First structural insight into lipid scrambling was provided from the X-ray structure of the fungal protein from Nectria haematococca, termed nhTMEM16. This protein is part of the TMEM16 family, which encompasses calcium-activated ion channels and lipid scramblases with a conserved molecular architecture. As common for the family, nhTMEM16 is a homodimer with subunits containing a cytoplasmic domain and a transmembrane unit composed of 10 membrane-spanning segments. The lipid permeation path is defined by a structural entity termed the ‘subunit cavity’, which is located at the periphery of each subunit. The ‘subunit cavity’ is believed to provide a pathway for the polar moieties of lipids across the membrane, whereas the apolar acyl chains remain embedded in the hydrophobic core of the bilayer.

The differences between structures of nhTMEM16 determined in detergents and in a lipid environment are most pronounced for the Ca2+-free state determined at 3.8 Å resolution. Whereas the structure in detergent displays a Ca2+-free conformation where the subunit cavity remains open to the membrane, the same region has changed its accessibility in the nanodisc sample. Here, the movement of α4 leads to a shielding of the cavity from the membrane core, resembling a conformation observed in the ion channel TMEM16A. This movement is accompanied by a conformational change of α6 as a consequence of the repulsion of negatively charged residues in the empty Ca2+-binding site. Generally, the Ca2+-free state of nhTMEM16 in nanodiscs is very similar to equivalent structures of its close homologs afTMEM16, TMEM16K and the more distantly related scramblase TMEM16F, thus underlining that all structures represent inactive conformations of the scramblase in the absence of ligand. Here, the Ca2+-free conformation obtained in nanodiscs defines a non-conductive state of the protein, where the polar subunit cavity is shielded from the membrane by tight interactions of α4 and α6 on the extracellular part of the membrane. The protein surface of the closed subunit cavity is hydrophobic as expected for a membrane protein. In this conformation, the Ca2+-binding site is empty, with the intracellular part of α6 positioned apart from the remainder of the binding site to release the electrostatic strain induced by the large negative net-charge in this region. Details of the conformation of α6 in the absence of Ca2+ differ between the family members of known structure with the conformation in nhTMEM16 being close to the one observed for TMEM16F.

>[2x]MSNLKDFSQPGSGQESNFGVDFVIHYKVPAAERDEAEAGFVQLIRALTTVGLATEVRHGENESLLVFVKVASPDLFAKQVYRARLGDWLHGVRVSAPHNDIAQALQDEPVVEAERLRLIYLMITKPHNEGGAGVTPTNAKWKHVESIFPLHSHSFNKEWIKKWSSKYTLEQTDIDNIRDKFGESVAFYFAFLRSYFRFLVIPSAFGFGAWLLLGQFSYLYALLCGLWSVVFFEYWKKQEVDLAVQWGVRGVSSIQQSRPEFEWEHEAEDPITGEPVKVYPPMKRVKTQLLQIPFALACVVALGALIVTCNSLEVFINEVYSGPGKQYLGFLPTIFLVIGTPTISGVLMGAAEKLNAMENYATVDAHDAALIQKQFVLNFMTSYMALFFTAFVYIPFGHILHPFLNFWRATAQTLTFSEKELPTREFQINPARISNQMFYFTVTAQIVNFATEVVVPYIKQQAFQKAKQLKSGSKVQEDHEEEAEFLQRVREECTLEEYDVSGDYREMVMQFGYVAMFSVAWPLAACCFLVNNWVELRSDALKIAISSRRPIPWRTDSIGPWLTALSFLSWLGSITSSAIVYLCSNSKNGTQGEASPLKAWGLLLSILFAEHFYLVVQLAVRFVLSKLDSPGLQKERKERFQTKKRLLQENLGQDAAEEAAAPGIEHSEKITREALEEEARQASIRGHGTPEEMFWQRQRGMQETIEIGRRMIEQQLAAGKNGKKSAPAVPSEKAS The CYP152 family of cytochrome P450 enzymes (P450s or CYPs) are bacterial peroxygenases that use hydrogen peroxide to drive hydroxylation and decarboxylation of fatty acid substrates. We have expressed and purified a novel CYP152 family member – CYP152K6 from the methylotroph Bacillus methanolicus MGA3. CYP152K6 is a previously uncharacterized member of the CYP152 P450 peroxygenase family which is able to hydroxylate at both the alpha and beta carbons on its fatty acid substrate. In contrast, the peroxygenase P450s have been shown to be efficient catalysts that convert fatty acids of various chain lengths to hydroxylated species and, for some of the peroxygenases, to terminal alkenes through an oxidative decarboxylation reaction.

However, CYP152K6 purified from an E. coli expression system was crystallized and its structure was determined to 1.3 Å with tetradecanoic acid bound. No lipids were present in conditions used for crystallogenesis, and thus CYP152K6 must form a complex by incorporating the fatty acid from E. coli cells. The protein crystallized with a single monomer in the asymmetric unit and showed good electron density for the entire protein molecule. An arginine residue, Arg244 in CYP152K6, is phylogenetically conserved in the CYP152 family of P450 peroxygenases, and makes strong hydrogen-bonding interactions with the carboxylate group of tetradecanoic acid. There are also extensive interactions made by several hydrophobic residues lining the active-site pocket that further stabilize the alkyl chain of tetradecanoic acid. The bound ligand is positioned in the active site in a binding mode that is above the plane of the heme, and with the Cα and Cβ carbons of tetradecanoic acid in close proximity of the heme iron (at distances of 4.8 Å and 5.5 Å, respectively). A water molecule at a distance of ~2.1 Å directly above the heme iron acts as the 6th (distal) ligand, with a cysteine thiolate providing the 5th (proximal) ligand. Interestingly, the distal water molecule is also within hydrogen-bonding distance (~3.0 Å) of one of the oxygen atoms from the carboxylate group of tetradecanoic acid. In contrast, the CYP152K6 tetradecanoic acid alkyl chain has a non-linear configuration in the active site. The alkyl chain bends by ~90° around the C8 atom of tetradecanoic acid to produce a well-defined structural “kink” in the lipid chain.

> GSMSNINQMPREEGIDSTWRLMEEGYMYILNRRHSFNSDIFETRLLGKKAICMGGKEAAEIFYDTEKFKRKDAAPNRVVQTLFGKNGVQALDGQTHKHRKEMFMSIMSPDELEKLTDITKKQWEIAVDKWEQMDKVILYEEAKEIMCRTACQWAGVPVQENEVKRLTKNLGAMFESAAAVGLKHWLGRHARNYEEIWIEELIDRVRDGKVNPPENTTLHKFSWYRDLEGNLLDTETAAVEVINILRPIVAIAIFINFIALALHHYPEEKEKLKSGDKKYSQMFVQEVRRFYPFFPFVVALVKKDFTWKGYKFEEGTLTLLDLYGTNHDPEIWKNPDVFSPDRFAKWEGSPFSFIPQGGGDYFMGHRCAGEWVTIEVMKVSLDYLTNRMDYEVPDQDLSFSMASMPSIPHSKVVIKNVKKRI[(2S,3R,4R,5S,6S)-2-[(3R,4R,5R,6R)-2-[(1R,2S)-2-[[6-amino-2-[(1S)-3-amino-1-[(2,3-diamino-3-oxopropyl)amino]-3-oxopropyl]-5-methylpyrimidine-4-carbonyl]amino]-3-[[(2S,3R,4R)-5-[[(2R,3S)-1-[2-[4-[4-[3-[4-(3-aminopropylamino)butylamino]propylcarbamoyl]-1,3-thiazol-2-yl]-1,3-thiazol-2-yl]ethylamino]-3-hydroxy-1-oxobutan-2-yl]amino]-3-hydroxy-4-methyl-5-oxopentan-2-yl]amino]-1-(3H-imidazol-4-yl)-3-oxopropoxy]-4,5-dihydroxy-6-(hydroxymethyl)oxan-3-yl]oxy-3,5-dihydroxy-6-(hydroxymethyl)oxan-4-yl] 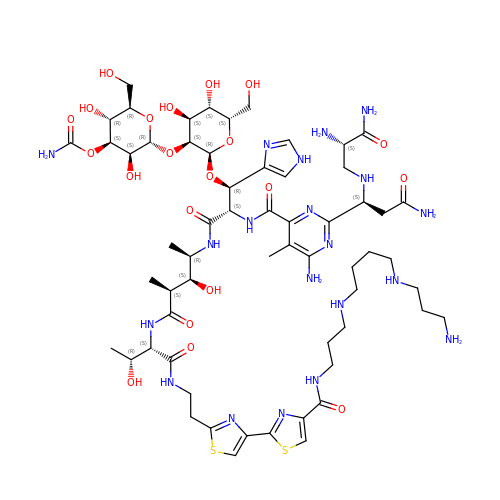carbamate | C60 H96 N20 O21 S2 | FOUFFVYWFNBHHH-YNGSZULRSA-N> DEELEDSKALLYLPIAPEVEDPEENPYGPPPDGSQPPKKKPKTTNIELQGVPNDEVHPLLGVK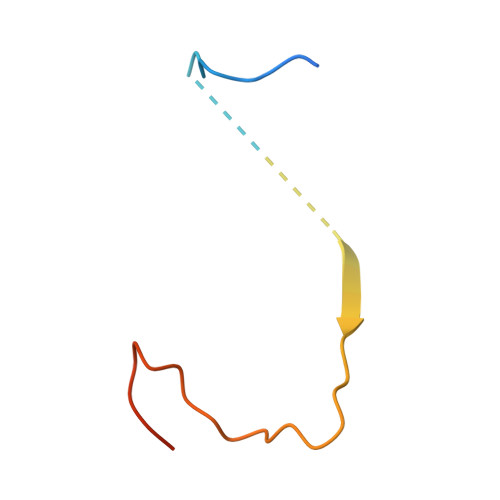GDGKSK>[2x]M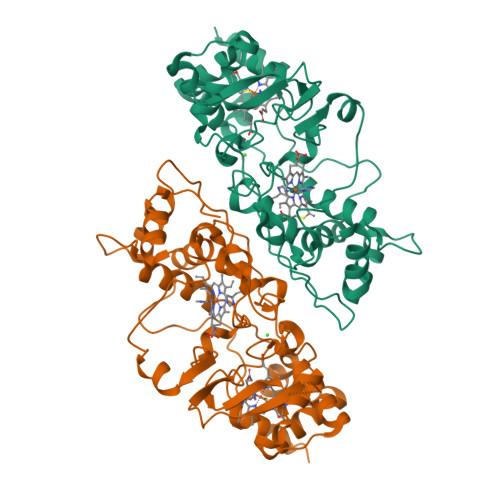KQLSVSLAILCAVATSEAFAADELQQRAQGLFKPVPAKAPTLKGNPASPVKVELGKMLYFDPRLSASHLISCNTCHNVGLGGGDLQATSTGHGWQKGPRNAPTVLNSVFNTAQFWDGRAKDLAEQAKGPVQAPKEMNNTPDQVVKTLNSIPDYVALFKKAFPGEKDPVTFDNMAKAIEVFEATLITPDSPFDQYLKGKKKALDGKQTAGLKLFLDKGCVACHGGLNLGGTGYFPFGVVEKPAENILPLGDKGRFAVTNTAKDEYVFRAPSLRNVAITYPYFHSGVVWSLKEAVAVMGSAQFGIKLSDDESEAIAAFLGSLTGKQPKVVYPIMPASTDATPRPRL>CGCGAANT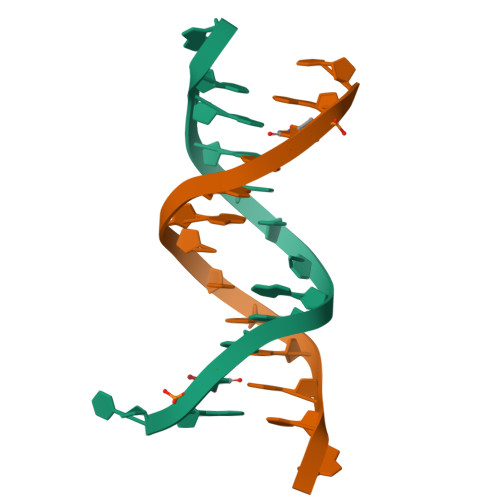TCGCG[12x]> MQNAGSLVVLGSINADHILNLQSFPTPGETVTGNHYQVAFGGKGANQAVAAGRSGANIAFIACTGDDSIGESVRQQLATDNIDITPVSVIKGESTGVALIFVNGEGENVIGIHAGANAALSPALVEAQRERIANASALLMQLESPLESVMAAAKIAHQ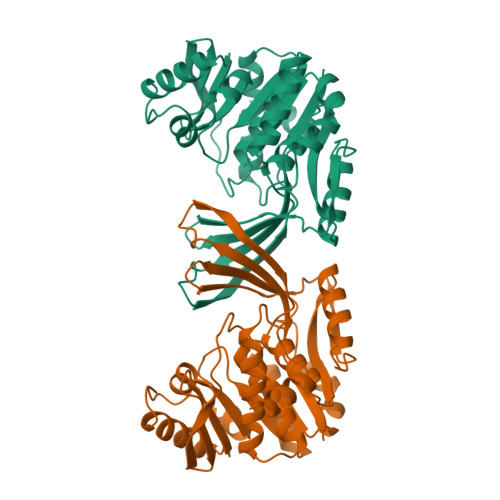NKTIVALNPAPARELPDELLALVDIITPNETEAEKLTGIRVENDEDAAKAAQVLHEKGIRTVLITLGSRGVWASVNGEGQRVPGFRVQAVDTIAAGDTFNGALITALLEEKPLPEAIRFAHAAAAIAVTRKGAQPSVPWREEIDAFLDRQR> SMSSSQSRSGGERMIHQDYIARIRYSNALPPPP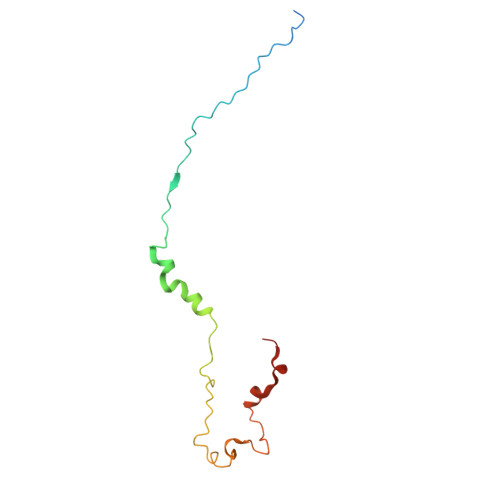IPPKLLDIPNTGLASGQYTAPGFASRLAREQPLNIEADAELGMPLDLVGMPGVFDGDESSIQAPAQPPPVHPHDRPLLRPLSTLGKPK>FTLIELMVVIGIIAILSAIGIPAYQNYLRKAALTDMLQTFVPYRTAVELCALEHGGLDTCDGGSNGIPSPTTTRYVSAMSVAKGVVSLTGQESLNGLSVVMTPGWDNANGVTGWARNCNIQSDSALQQACEDVFRFDDAN[14x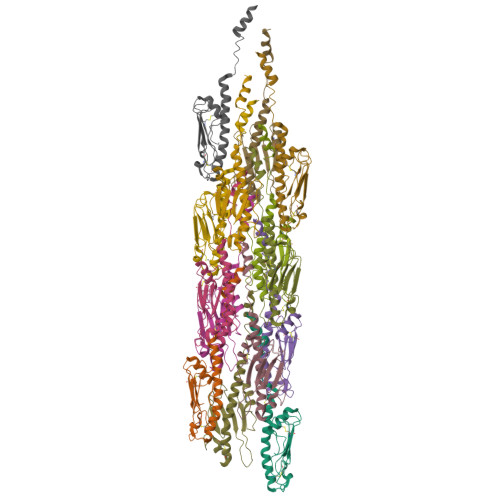]>MELWLVRHGETLWNREGRLLGWTDLPLTAEGEAQARRLKGALPSLPAFSSDLMRARRTAELAGFSPRLYPELREIHFGALEGALWETLDPRYKEALLRFQGFHPPGGESLSAFQERVFRFLE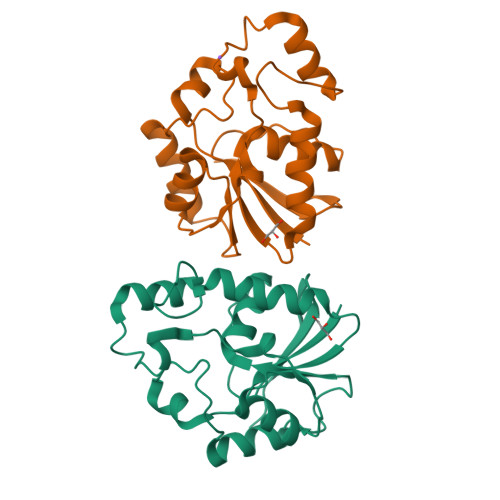GLKAPAVLFTHGGVVRAVLRALGEDGLVPPGSAVAVDWPRRVLVRLALDGEEATG[2x]>AAPDEITTAWPVNVGPLNPHLYTPNQMFAQSMVYEPLVKYQADGSVIPWLAKSWTHSEDGKTWTFTLRDDVKFSNGEPFDAEAAAENFRAVLDNRQRHAWLELANQIVDVKALSKTELQITLKSAYYPFLQELALPRPFRFIAPSQFKNHETMNGIKAPIGTGPWILQESKLNQYDVFVRNENYWGEKPAIKKITFNVIPDPTTRAVAFETGDIDLLYGNEGLLPLDTFARFSQNPAYHTQLSQPIETVMLALNTAKAPTNELAVREALNYAVNKKSLIDNALYGTQQVADT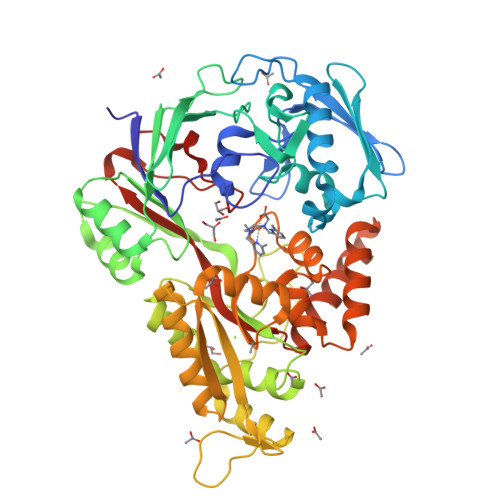LFAPSVPYANLGLKPSQYDPQKAKALLEKAGWTLPAGKDIREKNGQPLRIELSFIGTDALSKSMAEIIQADMRQIGADVSLIGEEESSIYARQRDGRFGMIFHRTWGAPYDPHAFLSSMRVPSHADFQAQQGLADKPLIDKEIGEVLATHDETQRQALYRDILTRLHDEAVYLPISYISMMVVSKPELGNIPYAPIATEIPFEQIKPVKP[2x]>[8x]MSQHNEKNPHQHQSPLHDSSEAKPGMDSLA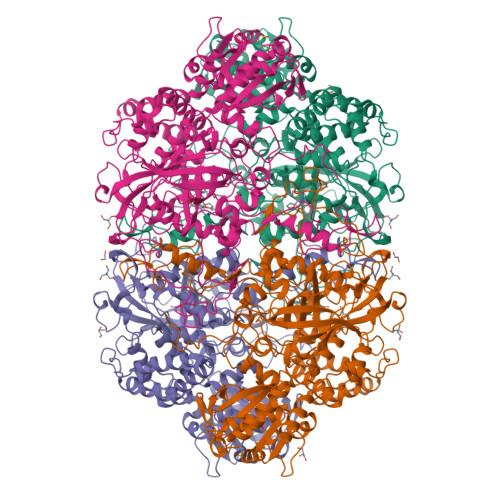PEDGSHRPAAEPTPPGAQPTAPGSLKAPDTRNEKLNSLEDVRKGSENYALTTNQGVRIADDQNSLRAGNRGPTLLEDFILREKITHFDHERIPERIVHARGSAAHGYFQPYKSLSDITKADFLSDPNKITPVFVRFSTVQGGAGSADTVRDIRGFATKFYTEEGIFDLVGNNTPIFFIQDAHKFPDFVHAVKPEPHWAIPQGQSAHDTFWDYVSLQPETLHNVMWAMSDRGIPRSYRTMEGFGIHTFRLINAEGKATFVRFHWKPLAGKASLVWDEAQKLTGRDPDFHRRELWEAIEAGDFPEYELGFQLIPEEDEFKFDFDLLDPTKLIPEELVPVQRVGKMVLNRNPDNFFAENEQAAFHPGHIVPGLDFTNDPLLQGRLFSYTDTQISRLGGPNFHEIPINRPTCPYHNFQRDGMHRMGIDTNPANYEPNSINDNWPRETPPGPKRGGFESYQERVEGNKVRERSPSFGEYYSHPRLFWLSQTPFEQRHIVDGFSFELSKVVRPYIRERVVDQLAHIDLTLAQAVAKNLGIELTDDQLNITPPPDVNGLKKDPSLSLYAIPDGDVKGRVVAILLNDEVRSADLLAILKALKAKGVHAKLLYSRMGEVTADDGTVLPIAATFAGAPSLTVDAVIVPCGNIADIADNGDANYYLMEAYKHLKPIALAGDARKFKATIKIADQGEEGIVEADSADGSFMDELLTLMAAHRVWSRIPKIDKIPA> SMPRITENIETYVTHLLSDLEPVPSQNQHLAYGYPGERQVFKDPMLDGKQVVVVNSQYDKHGRPVTGQPDVIQEANNYIDNLVAAAKSLIDKDKKGEKDLRKNAIDEMAKTFKKSISETIPSDKAKADLFSSKKSSANKDFLEQLAKVEGSLQQFTQAVAKASGHKLKALDKEGHNIRSHNRDTLIHRFKAPNSKEGEEQFIMYIPCGRYTKRQQRLMGKDESEVNRDHDTTSHKRSDLVLGNSSMARMIAGTRHSDGTVTIHHDSFSGPGARMPYSDFKGADDYKKLAIKAVTLINQEEVIQTLAQRQIDRMTNEDLWNKIPEEYRPDELPPDAEKARAQLIKLYVEHNPLSVTECYTQVVTAGQRVAAENQKEQFEYVRQMMDAFDGSKAKITIQTGSNTEVETAVGYQARMSSWGVNWFRQVGALNPLSDNSVTKNQNARFVNQMTDDVIRNLDKVAQNLGDYDKAGA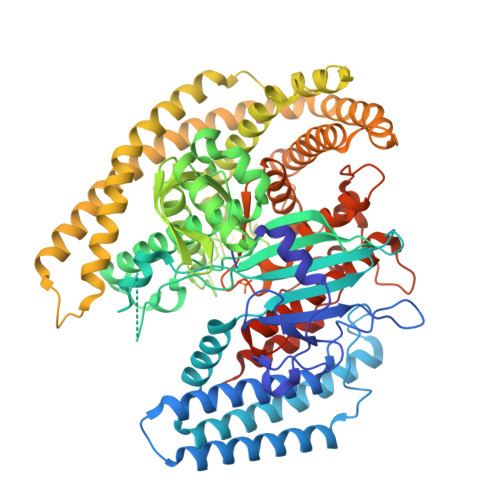LHTLLKGPDVSDLNQQITEKENALKEVKGAYREALFSYFEEYQKGEGKWDQAKLDQLKNQVDGYEKSIKKQESAIYELHNQIDALRKAYYTEHKGQINKALQELKEQISPVIQNKETDPETKSRLQHFYNSCAYLTQAQELYYENTWHHGKNNFKLQTLMASLSCELDYANTKGSKSNNDRGQRLAQKIVGNALWTAMSEDGLYTGEFLDHRRTHGKEVSNVEQLDRELTTIQALHHTANTGVSGGKFEIQDKANFADNGLFGKVANFAKIKEMGPENAFTKNMGTKIKA>[4x]NSVSMIGKIAETDVSGANFDGNNKLSFSLFFDEKIDASKGVPAIQILNENNELVKTIPLKDYNGQKGYINFEWDGTNEKGEKVPKGN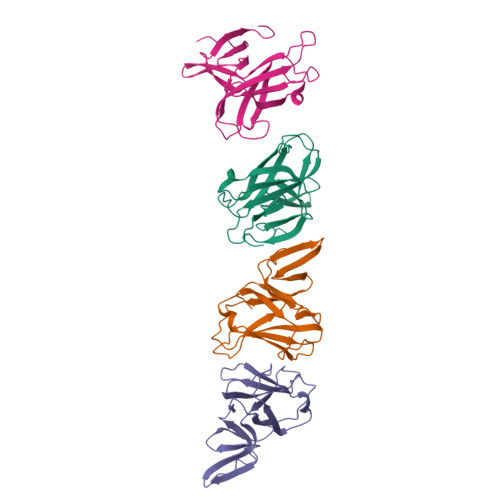YKIKAEYNLDSHSKQYLQTRIGRGEVESVIFDKGKPMLRMGEMILPIDSAIEFYKPDQK>MSDKDSKNTPQVPEKLGLSRRGFLGASAVTGAAVAATALGGAVMTRESWAQAVKESKQKIHVGPGELDDYYGFWSGGHQGEVRVLGVPSMRELMRIPVFNVDSATGWGLTNESRHIMGDSAKFLNGDCHAPHISMTDGKYDGKYLFINDKANSRVARIRLDIMKCDKMITVPNVQAIHGLRLQKVPHTKYVFANAEFIIPHPNDGKVFDLQDENSYTMYNAIDAETMEMAFQVIVDGNLDNTDADYTGRFAAATCYNSEKAFDLGGMMRNERDWVVVFDIHAVEAAVKAGDFITLGDSKTPVLDGRKKDGKDSKFTRYVPVPKNPHGCNTSSDGKYFIAAGKLSPTCSMIAIDKLPDLFAGKLADPRDVIVGEPELGLGPLHTTFDGRGNAYTTLFIDSQVVKWNMEEAVRAYKGEKVNYIKQKLDVHYQPGHLHASLCETNEADGKWLVALSKFSKDRFLPVGPLHPENDQLIDISGDEMKLVHDGPTFAEPHDCIMARRDQIKTKKIWDRNDPFFAPTVEMAKKDGINLDTDNKVIRDGNKVRVYMTSMAPAFGVQEFTVKQG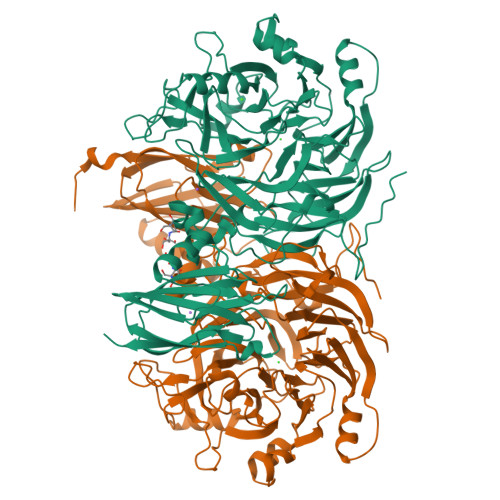DEVTVTITNIDQIEDVSHGFVVVNHGVSMEISPQQTSSITFVADKPGLHWYYCSWFCHALHMEMVGRMMVEPAWSHPQFEK[2x]> ADYDLKFGMNAGTSSNEYKAAEMFAKEVKEKSQGKIEISLYPSSQLGDDRAMLKQLKDGSLDFTFAESARFQLFYPEAAVFALPYVISNYNVAQKALFDTEFGKDLIKKMDKDLGVTLLSQAYNGTRQTTSNRAINSIADMKGLKLRVPNAATNLAYAKYVGASPTPMAFS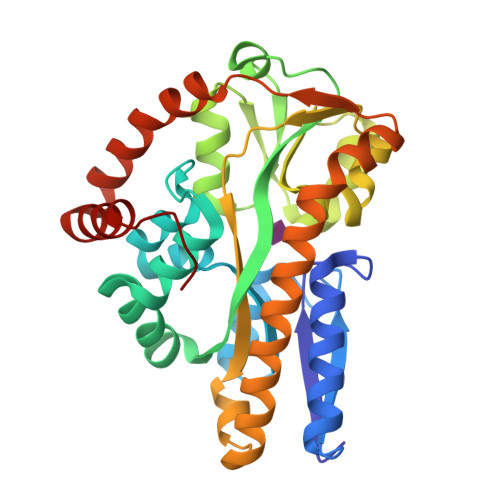EVYLALQTNAVDGQENPLAAVQAQKFYEVQKFLAMTNHILNDQLYLVSNETYKELPEDLQKVVKDAAENAAKYHTKLFVDGEKDLVTFFEKQGVKITHPDLVPFKESMKPYYAEFVKQTGQKGESALKQIEAINPKGEA>[6x]MLDSKLKAPVFTVRTQGREYGEFVLEPLERGFGVTLGNPLRRILLSSIPGTAVTSVYIEDVLHEFSTIPGVKEDVVEIILNLKELVVRFLNPSLQTVTLLLKAEGPKEVKARDFLPVADVEIMNPDLHIATLEEGGRLNMEVRVDRGVGYVPAEKHGIKDRINAIPVDAVFSPVRRVAFQVEDTRLGQRTDLDKLTLRIWTDGSVTPLEALNQAVEILREHLTYFSNPQAAAVAAPEEAKEPEAPPEQEEELDLPLEELGLSTRVLHSLKEEGIESVRALLALNLKDLKNIPGIGERSLEEIKEALEKKGFTLKE;>MEIKRFGRIREVIPLPPLTEIQVESYRRALQADVPPEKRENVGIQAAFRETFPIEEEDKGKGGLVLDFLEYRLGEPPFPQDECREKDLTYQAP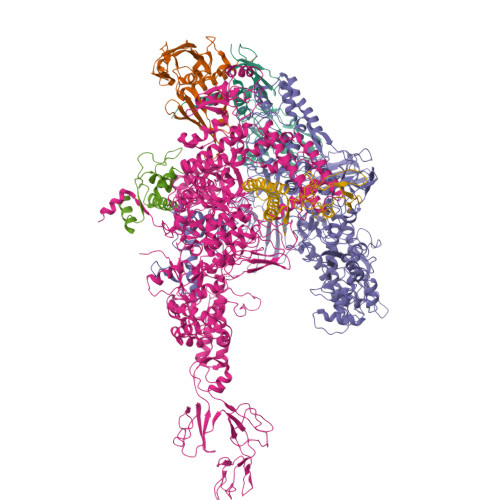LYARLQLIHKDTGLIKEDEVFLGHIPLMTEDGSFIINGADRVIVSQIHRSPGVYFTPDPARPGRYIASIIPLPKRGPWIDLEVEPNGVVSMKVNKRKFPLVLLLRVLGYDQETLARELGAYGELVQGLMDESVFAMRPEEALIRLFTLLRPGDPPKRDKAVAYVYGLIADPRRYDLGEAGRYKAEEKLGIRLSGRTLARFEDGEFKDEVFLPTLRYLFALTAGVPGHEVDDIDHLGNRRIRTVGELMTDQFRVGLARLARGVRERMLMGSEDSLTPAKLVNSRPLEAAIREFFSRSQLSQFKDETNPLSSLRHKRRISALGPGGLTRERAGFDVRDVHRTHYGRICPVETPEGANIGLITSLAAYARVDELGFIRTPYRRVVGGVVTDEVVYMTATEEDRYTIAQANTPLEGNRIAAERVVARRKGEPVIVSPEEVEFMDVSPKQVFSVNTNLIPFLEHDDANRALMGSNMQTQAVPLIRAQAPVVMTGLEERVVRDSLAALYAEEDGEVAKVDGNRIVVRYEDGRLVEYPLRRFYRSNQGTALDQRPRVVVGQRVRKGDLLADGPASENGFLALGQNVLVAIMPFDGYNFEDAIVISEELLKRDFYTSIHIERYEIEARDTKLGPERITRDIPHLSEAALRDLDEEGVVRIGAEVKPGDILVGRTSFKGESEPTPEERLLRSIFGEKARDVKDTSLRVPPGEGGIVVRTVRLRRGDPGVELKPGVREVVRVYVAQKRKLQVGDKLANRHGNKGVVAKILPVEDMPHLPDGTPVDVILNPLGVPSRMNLGQILETHLGLAGYFLGQRYISPIFDGAKEPEIKELLAQAFEVYFGKRKGEGFGVDKREVEVLRRAEKLGLVTPGKTPEEQLKELFLQGKVVLYDGRTGEPIEGPIVVGQMFIMKLYHMVEDKMHARSTGPYSLITQQPLGGKAQFGGQRFGEMEVWALEAYGAAHTLQEMLTLKSDDIEGRNAAYEAIIKGEDVPEPSVPESFRVLVKELQALALDVQTLDEKDNPVDIFEGLASKR[3x];>MKKEVRKVRIALASPEKIRSWSYGEVEKPETINYRTLKPERDGLFDERIFGPIKDYECACGKYKRQRFEGKVCERCGVEVTKSIVRRYRMGHIELATPAAHIWFVKDVPSKIGTLLDLSATELEQVLYFSKYIVLDPKGAILNGVPVEKRQLLTDEEYRELRYGKQETYPLPPGVDALVKDGEEVVKGQELAPGVVSRLDGVALYRFPRRVRVEYVKKERAGLRLPLAAWVEKEAYKPGEILAELPEPYLFRAEEEGVVELKELEEGAFLVLRREDEPVATYFLPVGMTPLVVHGEIVEKGQPLAEAKGLLRMPRQVRAAQVEAEEEGETVYLTLFLEWTEPKDYRVQPHMNVVVPEGARVEAGDKIVAAIDPEEEVIAEAEGVVHLHEPASILVVKARVYPFEDDVEVSTGDRVAPGDVLADGGKVKSDVYGRVEVDLVRNVVRVVESYDIDARMGAEAIQQLLKELDLEALEKELLEEMKHPSRARRAKARKRLEVVRAFLDSGNRPEWMILEAVPVLPPDLRPMVQVDGGRFATSDLNDLYRRLINRNNRLKKLLAQGAPEIIIRNEKRMLQEAVDALLDNGRRGAPVTNPGSDRPLRSLTDILSGKQGRFRQNLLGKRVDYSGRSVIVVGPQLKLHQCGLPKRMALELFKPFLLKKMEEKGIAPNVKAARRMLERQRDIKDEVWDALEEVIHGKVVLLNRAPTLHRLGIQAFQPVLVEGQSIQLHPLVCEAFNADFDGDQMAVHVPLSSFAQAEARIQMLSAHNLLSPASGEPLAKPSRDIILGLYYITQVRKEKKGAGLEFATPEEALAAHERGEVALNAPIKVAGRETSVGRLKYVFANPDEALLAVAHGIVDLQDVVTVRYMGKRLETSPGRILFARIVAEAVEDEKVAWELIQLDVPQEKNSLKDLVYQAFLRLGMEKTARLLDALKYYGFTFSTTSGITIGIDDAVIPEEKKQYLEEADRKLLQIEQAYEMGFLTDRERYDQILQLWTETTEKVTQAVFKNFEENYPFNPLYVMAQSGARGNPQQIRQLCGLRGLMQKPSGETFEVPVRSSFREGLTVLEYFISSHGARKGGADTALRTADSGYLTRKLVDVTHEIVVREADCGTTNYISVPLFQPDEVTRSLRLRKRADIEAGLYGRVLAREVEVLGVRLEEGRYLSMDDVHLLIKAAEAGEIQEVPVRSPLTCQTRYGVCQKCYGYDLSMARPVSIGEAVGIVAAQSIGEPGTQLTMRTFHTGGVAGAADITQGLPRVIELFEARRPKAKAVISEIDGVVRIEETEEKLSVFVESEGFSKEYKLPKEARLLVKDGDYVEAGQPLTRGAIDPHQLLEAKGPEAVERYLVEEIQKVYRAQGVKLHDKHIEIVVRQMMKYVEVTDPGDSRLLEGQVLEKWDVEALNERLIAEGKTPVAWKPLLMGVTKSALSTKSWLSAASFQNTTHVLTEAAIAGKKDELIGLKENVILGRLIPAGTGSDFVRFTQVVDQKTLKAIEEARKEAVEAKERPAARRGVKREQPGKQA[3x];>MAEPGIDKLFGMVDSKYRLTVVVAKRAQQLLRHGFKNTVLEPEERPKMQTLEGLFDDPNAVTWAMKELLTGRLVFGENLVPEDRLQKEMERLYPVEREE[3x];>[3x]MAREVKLTKAGYERLMQQLERERERLQEISADFEQALEEGDLRENAGYDEARRAMWQNEARIDSLEDILSRAVILEEGSGEVIGLGSVVELEDPLSGERLSVQVVSPAEANVLDTPMKISDASPMGKALLGHRVGDVLSLDTPKGRREFRVVAIHG> MDLYAVWGNPIAQSKSPLIQNKLAAQTHQTMEYIAKLGDLDAFEQQLLAFFEEGAKGCNITSPFKERAYQLADEYSQRAKLAEACNTLKKLDDGKLYADNTDGIGLVTDLQRLNWLRPNQHVLILGAGGATKGVLLPLLQAQQNIVLANRTFSKTKELAERFQPYGNI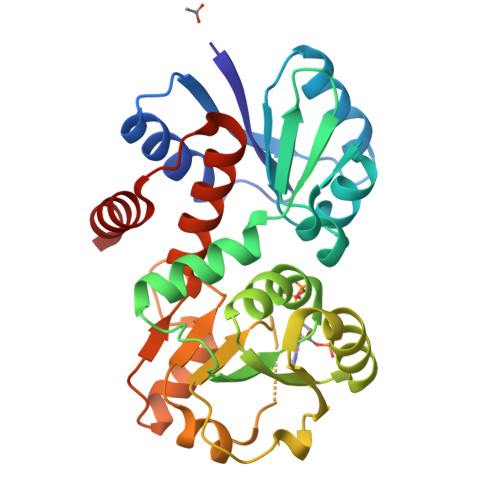QAVSMDSIPLQTYDLVINATSAGLSGGTASVDAEILKLGSAFYDMQYAKGTDTPFIALCKSLGLTNVSDGFGMLVAQAAHSFHLWRGVMPDFVSVYEQLKKAML>[3x]GCS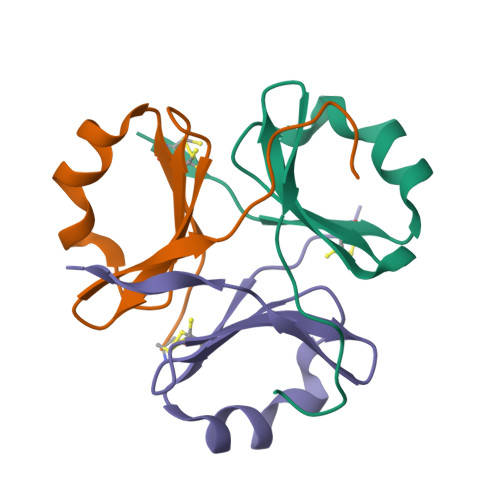SGVRCWATRQAMLGQVHEVPEGWLIFVAEQEELYVRVQNGFRKVQLEARTPLPR> MISLNGYGRFGLQYVEDRGVGLEDTIISSRLRINIVGTTETDQGVTFGAKLRMQWDDGDAFAGTAGNAAQFWTSYNGVTVSVGNVDTAFDSVALTYDSWMGYEASSFGDAQSSFFWYNSKYDASGALDNYNGIAVTYSISGVNLYLSYVDPDQTVDSSLVTEEFGIAADWSNDMISLAAAYTTDAGGIVDNDIAFVGAAYKFNDAGTVGLNW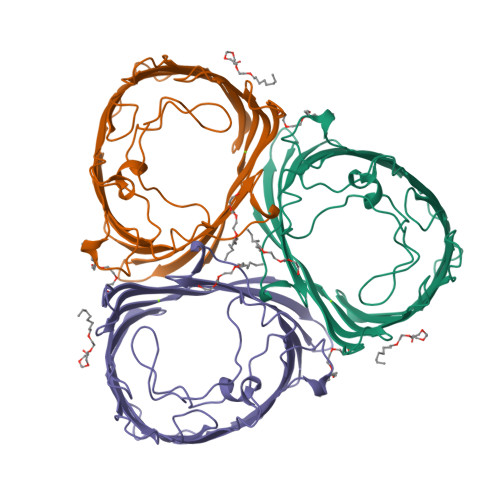YDNGLSTAGDQVTLYGNYAFGATTVRAYVSDIDRAGADTAYGIGADYQFAEGVKVSGSVQSGFANETVADVGVRFDF> MFRVTGLQLKNPVVFKQGQGMFSHQLKRLLQKKSIHRYNWDPLPMYDPRKLVHASRHMDVETWREVPDPHWDE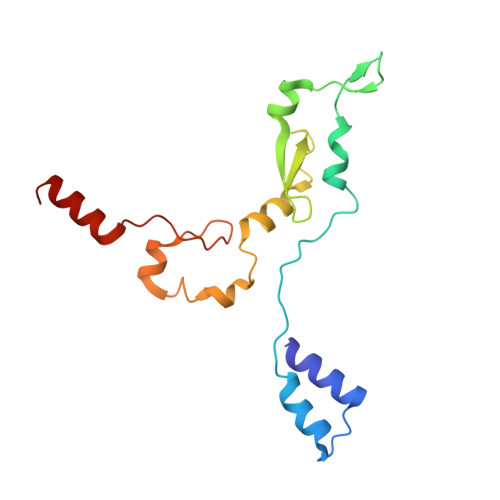RSYLVPDQMFYNIPVPPEYKDAYWWRELQARRVQCPVEWVSHRMYNKGDRQRYDFQDLAFRKKFEFSYEEVVKNAKDMRS Self-labeling protein tags such as HaloTag are powerful tools that can label fusion proteins with synthetic fluorophores for use in fluorescence microscopy. Here we introduce HaloTag variants with either increased or decreased brightness and fluorescence lifetime compared with HaloTag7 when labeled with rhodamines. To engineer the binding site, ten amino acids on helices 6–8 in close proximity to TMR were chosen for randomization by site-saturation mutagenesis. The changes in spectroscopic properties result from single or double point mutations in the direct vicinity of the bound fluorophore.

The brightest variant, the double mutant HaloTag9 (HaloTag7-Q165H-P174R, ΔI = 19.9 ± 0.5%), as well as the dimmer variants HaloTag10 (HaloTag7-Q165W, ΔI = −52.9 ± 1.2%) and HaloTag11 (HaloTag7-M175W, ΔI = −44.8 ± 0.8%) were chosen for characterization with a panel of 46 different fluorophores and analysis of their photophysical properties. HaloTag10 and HaloTag11 decreased the fluorescence intensity of almost all tested fluorophores compared with HaloTag7. The decreases were more pronounced for HaloTag10 than for HaloTag11 but in both cases caused by changes in quantum yield. For HaloTag10 and HaloTag11, the proximity of TMR to the introduced tryptophans suggests that photoinduced electron transfer (PET) quenching of the fluorophore is responsible for the decreased quantum yields. The decreased quantum yields and fluorescence lifetimes of HaloTag10 and HaloTag11 presumably result from PET quenching through the newly introduced tryptophans. HaloTag10 and HaloTag11 decreased the brightness of all fluorophores relative to HaloTag7, HaloTag10 having the biggest effect. Photostability measurements showed that the higher the fluorescence lifetime, the more photobleaching occurred, making HaloTag9 the least and HaloTag10 and HaloTag11 the most photostable tags. We therefore recommend the use of HaloTag9 and HaloTag11 for multiplexing of two species and HaloTag9, HaloTag10 and HaloTag11 for multiplexing of three species.

>GIGTGFPFDPHYVEVLGERMHYVDVGPRDGTPVLFLHGNPTSSYVWRNIIPHVAPTHRCIAPDLIGMGKSDKPDLGYFFDDHVRFMDAFIEALGLEEVVLVIHDWGSALGFHWAKRNPERVKGIAFMEFIRPIPTWDEWPEFARETFQAFRTTDVGRKLIIDQNVFIEGTLPWGVVRPLTEVEMDHYREPFLNPVDREPLWRFPNELPIAGEPANIVALVEEYMDWLHQSPVPKLLFWGTPGVLIPPAEAARLAKSLPNCKAVDIGPGLNLLQEDNPDLIGSEIARWLSTLEI[4x]>RSYSNRTLPDTVDWREKGCVTEVKYQGSCGACWAFSAVGALEGQLKLKTGKLISLSAQNLVDCSNEEKYGNKGCGGGYMTEAFQYIIDNGGIEADASYPYKAMDEKCHYNSKNRAATCSRYIQLPFGDEDALKEAVATKGPVSVGIDASHSSFFFYKSGVYDDPSCTGNVNHGVLVVGYGTLDGKDYWLVKNSWGLNFGDQGYI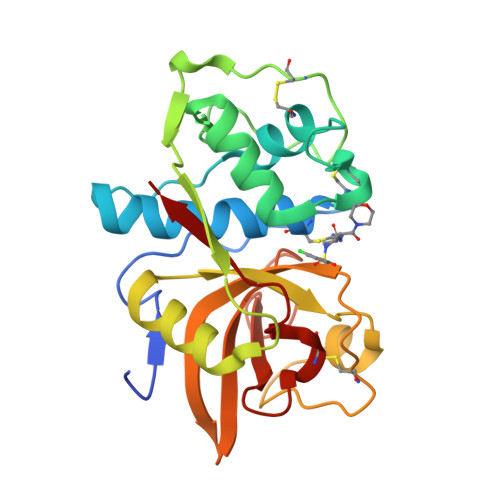RMARNNKNHCGIASYCSYPEI[2x]> MWGGGKMAVVSLSPHTAKMRKLFGQASTTMAYDGLKREAERRTRSDHNITMVAKDDELYLYHLTLKKQTNFVHSCIGHFVDLEAGSKREQSQLCVATETHLELYDTADGELKLIAKFQNLFATITSMKSLDLPHSGSRAKASNWPTFLALTSDSGNLSIVQIIMHAGALRLKTLVNQPLTRTTLRRVSPISYMEIDPNGRCIILSSVEQNKLCFLVDYAQKLRISSPLEIIRPHMVTLDMAVVDVNFNNPCFVTLEIDNAATQLSVHLIFYVLELGLNHIVKKADYLVNPSANFVLSLPDLSRYNITTSLSDNNYDADYDTLFNPFVVIGFENHILVKDMNGFFSLKVEIPKRSITNSRHKNVTIISGIVQKLKNDFFVLLQSNHGDLFKLTVSPDTNDRNRPLVQLSYFDTIQNSHQLHIFKNGYLFALSEMNNNFLFQFEKLGVEKNDFSNVLTSKDPNKSLVFEPSIKLQNLSILSQQLNLNPSIKSQIVSDSPLSIATKHFTNNKIITLTNAVNYSNLISTSLPPNATKLWLIPDPATTGDNNTLLFITFPKKTMILQIDNESMEELTPDEATRSAFKLSQDTTIHTCLMGSHSIIQVCTAELRHIVPTGKSRYSNKLTWVPPAGIRIVCATSSKTQLIISLSNYELVYFKIDVSSDSLIELTTHPELDTMPSKVAIVQDTQHADLLAIADNEGMIKIMSLKDQKEDFLTVISLQLVSEKISDMIMVRDSSIGQLNLHVGLENGVYMKF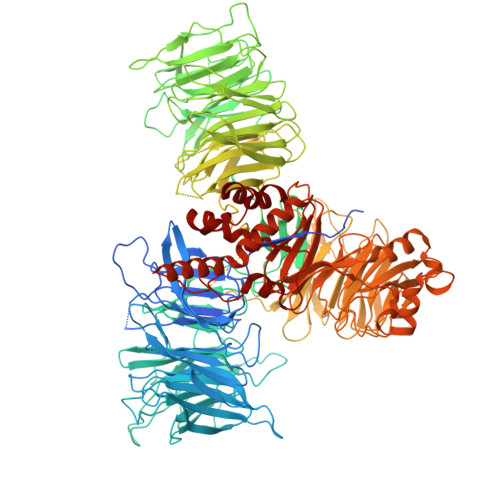HIGDVDGSFTDIKRRFLGLKPVSLSYLREISVSLNNEEEEEEEEDDDDEKEEEEINSSGAKWMSCVVCHSSSTWVSYTWKNVWTIRQLKDQNMLSCSKFVNADVAINGVCSISSSGRLNIGRVSNFPTLDNWFHVHESSVNKQENGGGDESNEEEEDEMEEEMEMLQISTFRPRTILSFPNNPKSILFIDNHSGKKQCRISLQIDGECLKFGSSDHLYKILDDIDCVSAAIIDFTRQADHLIICAGDKRLLTYKILVNKDKLSFDIELLHQTEIISPIHAMLKFKNFLLTAMGSTIVLYGLGKKQLLRRSVTQTPVSITKIVSMHQWNYERLAVGDIHESVTLFIWDPAGNVFIPYVDDSVKRHVTVLKFLDEATVIGADRYGNAWTLRSPPECEKIMSNHDPSELSNGAIKYPLDVITLQQKLPNTYDCKFKFQLLNHFFVNDIITDFHILDSLSNSDRPGCIYMGLQGTVGCFIPLLSKGNVFMMGNIENIMAEADDTFYLDYESRKKNNNMRKEDDEEESGSVVLQGRHGIEDEIICEGSCSILGRDHQEYRSYYAPVRKVIDGDLCENFLRLSLNEQEFLAKNLKSVQVEDIIQTINEVRTNYM> TCTGCGGT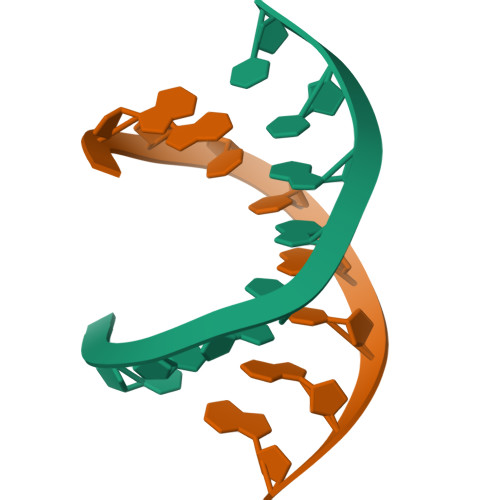C;> TGACCGCAG(3S)-3-hydroxybutyl 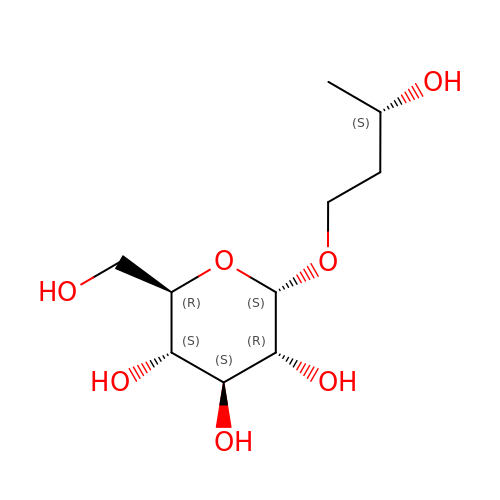alpha-D-glucopyranoside | C10 H20 O7 | IQTXPPTUXXJFDH-DLXYEPTOSA-N> GPLGSPEFPGRLEMEPDFYCVKWIPWKGEQTPIITQSTNGPCALLAIMN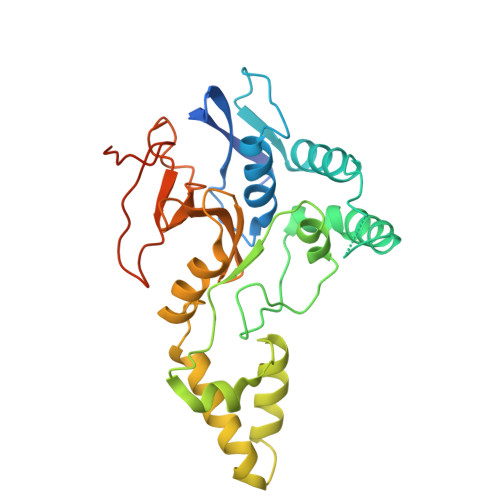ILFLQWKVKLPPQKEVITSDELMAHLGNCLLSIKPQEKSEGLQLNFQQNVDDAMTVLPKLATGLDVNVRFTGVSDFEYTPECSVFDLLGIPLYHGWLVDPQSPEAVRAVGKLSYNQLVERIITCKHSSDTNLVTEGLIAEQFLETTAAQLTYHGLCELTAAAKEGELSVFFRNNHFSTMTKHKSHLYLLVTDQGFLQEEQVVWESLHNVDGDSCFCDSDFHLSHSLGKGPGAEGGSGSPE> LDFDILTNDGTHRNMKLLIDLKNIFSRQLPKMPKEYIVKLVFDRHHESMVILKNKQKVIGGICFRQYKPQRFAEVAFLAVTANEQVRGYGTRLMNKFKDHMQKQNIEYLLTYADNFAIGYFKKQGFTK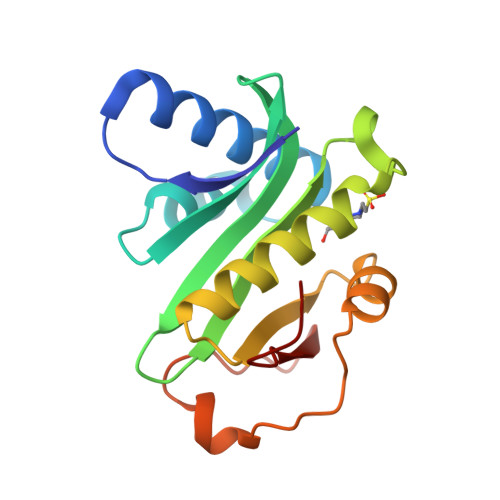EHRMPQEKWKGYIKDYDGGTLMECYIHPYVDY> MVDGNYSVASNVMVPMRDGVRLAVDLYRPDADGPVPVLLVRNPFDKFDVFAWSTQSTNWLEFVRDGYAVVIQDTRGLFASEGEFVPHVDDEADAEDTLSWILEQAWCDGNVGMFGVSYLGVTQWQAAVSGVGGLKAIAPSMASADLYRAPWYGPGGALSVEALLGWSALIGTGLITSRSDARPEDAADFVQLAAILNDVAGAASVTPLAEQPLLGRLIPWVIDQVVDHPDNDESWQSISLFERLGGLATPALITAGWYDGFVGESLRTFVAVKDNADARLVVGPWSHSNLTGRNADRKFGIAATYPIQEATTMHKAFFDRHLRGETDALAGVPKVRLFVMGIDEWRDETDWPLPDTAYTPFYLGGSGAANTSTGGGTLSTSISGTESADTYLYDPADPVPSLGGTLLFHNGDNGPADQRPIHDRDDVLCYSTEVLTDPVEVTGTVSARLFVSSSAVDTDFTAKLVDVFPDGRAIALCDGIVRMRYRETLVNPTLIEAGEIYEVAIDMLATSNVFLPGHRIMVQVSSSNFPKYDRNSNTGGVIAREQL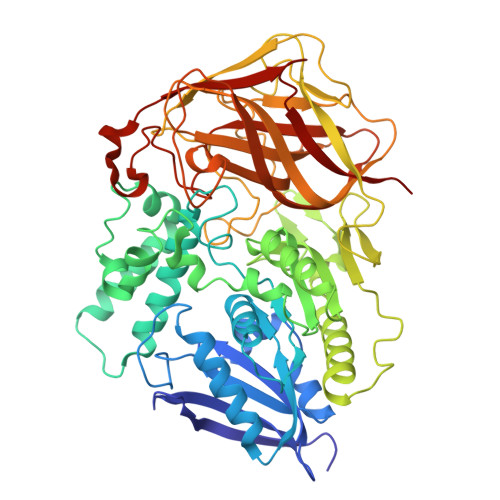EEMCTAVNRIHRGPEHPSHIVLPIIKR{3-[(3-HYDROXY-2-METHYL-5-PHOSPHONOOXYMETHYL-PYRIDIN-4-YLMETHYL)-AMINO]-2-METHYL-PROPYL}-PHOSPHONIC ACID | C11 H20 N2 O9 P2 | 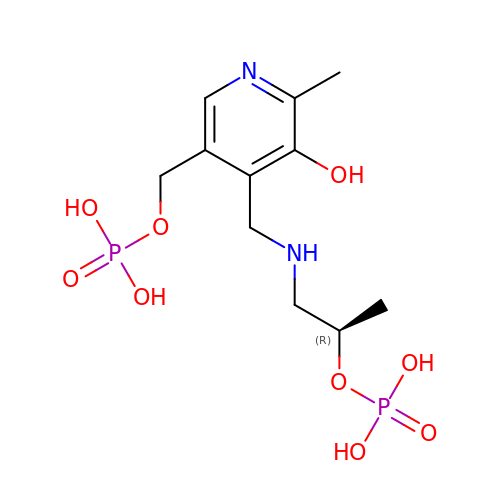JMZWWHLIKAYMPJ-SSDOTTSWSA-N>MVINMVDVIKFKEPERCDYLYVDENNKVHILLPIVGGDEIGLDNTCQTAVELITFFYGSAHSGVTKYSAEHQLSEYKRQLEEDIKAINSQKKISPHAYDDLLKEKIERLQQIEKYIELIQVLKKQYDEQNDIRQLRTGGIPQLPSGVKEIIKSSENAFAVRLSPYDNDKFTRFDDPLFNVKRNISKYDTPSRQAPIPIYEGLGYRLRSTLFPEDKTPTPINKKSLRDKVKSTVLSHYKDEDRIDGEKKDEKLNELITNLQNELVKELVKSDPQYSKLSLSKDPRGKEINYDYLVNSLMLVDNDSEIGDWIDTILDATVDSTVWAVQASSPFYQGAKEISSDRDADKISIRVQYLLAEANIYCKTNKLSDANFGEFFDKEPHATEIAKRVKEGFTQGADIEPIIYDYINSNHAELGLKSPLTGKQQQEITDKFTKHYNTIKESPHFDEFFVADPDKKGNIFSHQGRISCHFLDFFTRQTKGKHPLGDLASHQEALQEGTSNRLHHKNEVVAQGYEKLDQFKKEVVKLLAENKPKELLDYLVATSPTGVPNYSMLSKETQNYIAYNRNWPAIQKELEKATSIPESQKQDLSRLLSRDNLQHDNLSAITWSKYSSKPLLDVELNKIAEGLELTAKIYNEKRGREWWFAGSRNEARKTQCEELQRVSKEINTLLQSESLTKSQVLEKVLNSIETLDKIDRDISAESNWFQSTLQKEVRLFRDQLKDICQLDKYYFKSTKLDEIISLEMEEQFQKIQDPAVQQIVRDLPSHCHNDEAIEFFKTLNPEEAAKVASYLSL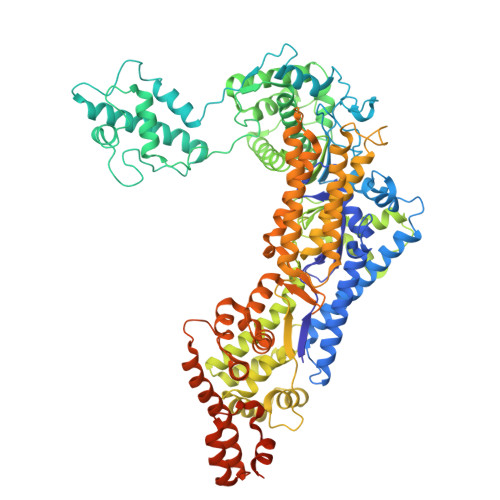EYREINKSTDKKTLLEQDIPRLFKEVNTQLLSKLKEEKAIDEQVHEKLSQLADKIAPEHFTRNNIIKWSTNPEKLEESNLNEPIKSVQSPTTKQTSKQFREAMGEITGRNEPPTDTLYTGIIKK[2x]>MKLSPKAATLAERSAGLAFSLYQAMAKDQAVENILLSPVVVASSLGLVSLGGKATTASQAKAVLSAEQLRDEEVHAGLGELLRSLSNSTARNVTWKLGSRLYGPSSVSFAEDFVRSSKQHYNCEHSKINFRDKRSALQSINEWAAQTTDGKLPEVTKDVERTDGALLVNAMFFKPHWDEKFHHKMVDNRGFMVTRSYTVGVTMMHRTGLYNYYDDEKEKLQIVEMPLAHKLSSLIILMPNNVEPLERLEKLLTKEQLKIWMGKMQKKAVAISLPKGVVEVTHDLQKHL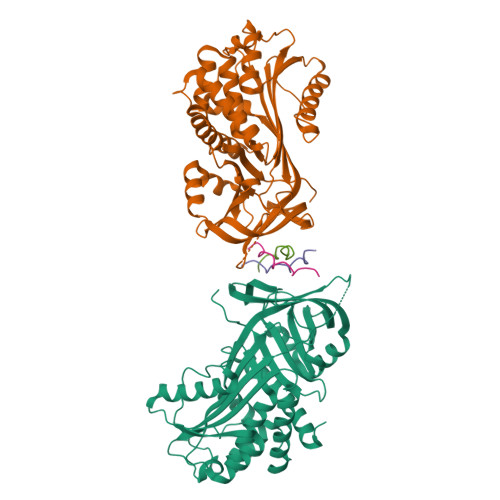AGLGLTEAIDKNKADLSRMSGKKDLYLASVFHATAFEWDTEGNPFDQDIYGREELRSPKLFYADHPFIFLVRDTQSGSLLFIGRLVRPKGDKMRDELLEHHHHHH[4x];>[6x]XPPGPPGPRGPPGPPGX4-[(5-bromopyridin-2-yl)amino]-4-oxobutanoic 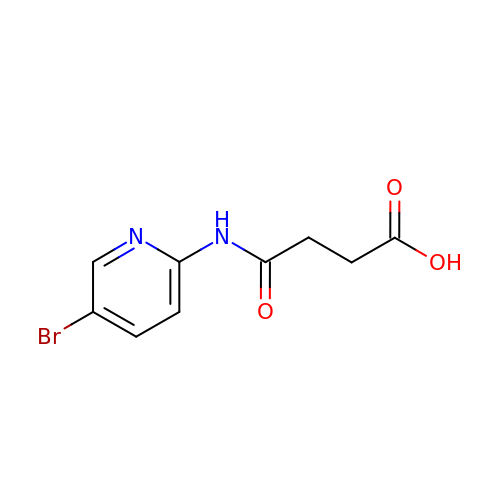acid | C9 H9 Br N2 O3 | XFYYQDHEDOXWGA-UHFFFAOYSA-N> MNSQYMFDYPAINIDVRCHRLLSSVSYVAYNKFHTHDVSTYEHCEIPLEKLRLGFGRRNSLADFYSLGELPASWGPACYFSSVKPM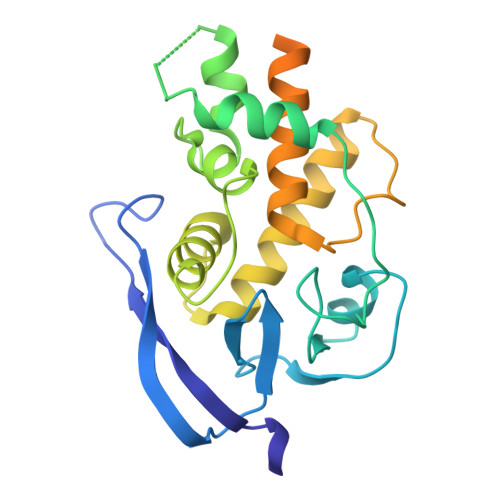MYTFQGMASDLSRFDLTSFSRKGLPNVLKALSWPLGIPDCEIFSICSDRFVRGLQTRDQLMSYILRMGDSHSLDECIVQAHKKILQEARRLGLSDEHYNGYDLFREIGSLVCLRLINAEPFDTASSGEALDVRTVIRSYRASDPSTGLTEYGNSLWTPIHSHVDENDESSSDSDF> NPYNKLFEERIIFLGVQVDDASANDIMAQLLVLESLDPDRDITMYINSPGGGFTSLMAIYDTMQYVRADIQTVCLGQAASAAAVLLAAGTPGKRMALPNARVLIHQPSLSGVIQGQFSDLEIQAAEIERMRTLMETTLARHTGKDAGVIRKDTDR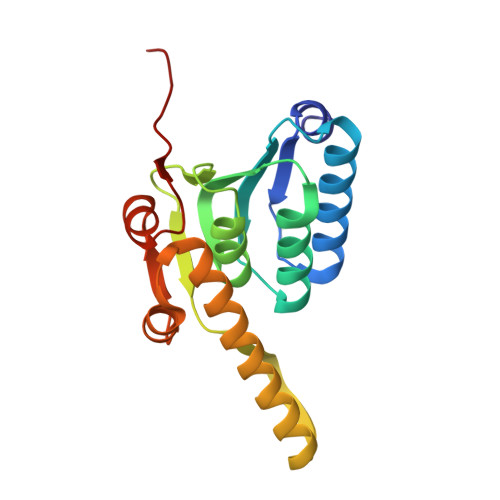DKILTAEEAKDYGIIDTVLEYRKLS>[4x]MPVFTIRTNVCRDSVPDTLLSDLTKQLAKATGKPAEYIAIHIVPDQIMSF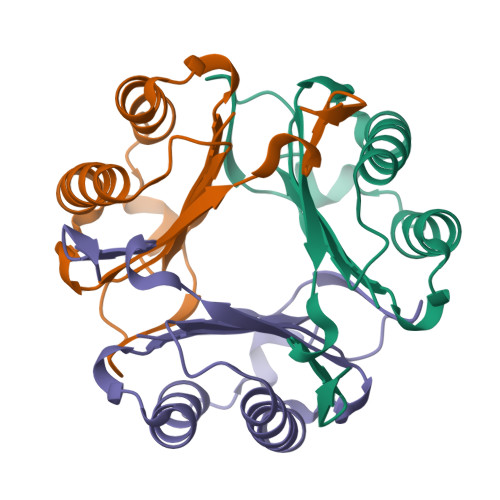GDSTDPCAVCSLCSIGKIGGPQNKSYTKLLCDILTKQLNIPANRVYINYYDLNAANVGWNGSTFA>MRGSHHHHHHGSGATRIQIALKYDEKNKQFAILIIQLSNLSALLQQQDQKVNIRVAVLPCSESTTCLFRTRPLDASDTLVFNEVFWVSMSYPALHQKTLRVDVCTTDRSHLEECLGGAQISLAEVARSGERSTR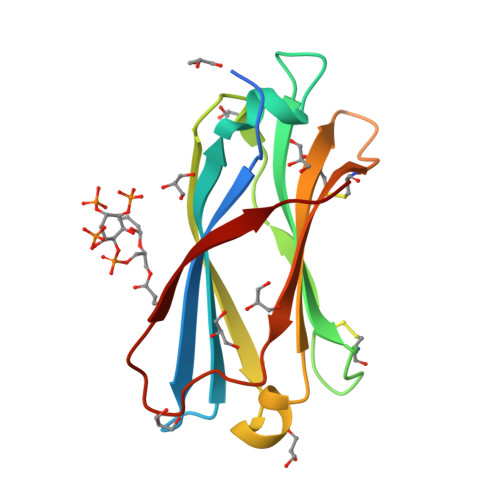WYNLLS[2x]>KAISYEQLSLASVGSVERLEGKIVGMNPPQFASINEFKYCTLKLYFTQLLPNVPDKVLVPGVNCIEIVIPTRERICELFGVLNCQSDKISDILLLEKPDRISVEVERILWDNDKTAS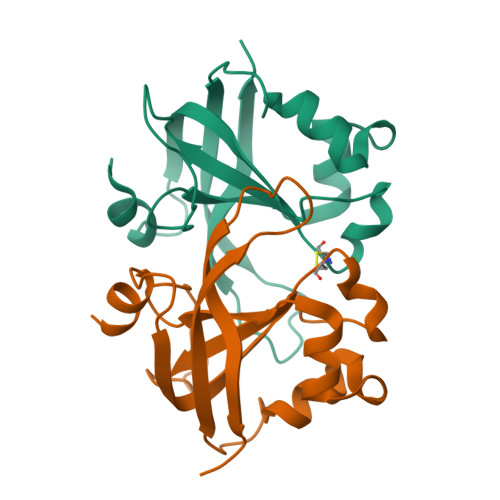PGMAVWSLKNISTDTQAQAQVQVPAQSSASIDPSR[2x]> SKALLKGVRDFNPISACVCLLENSSDGH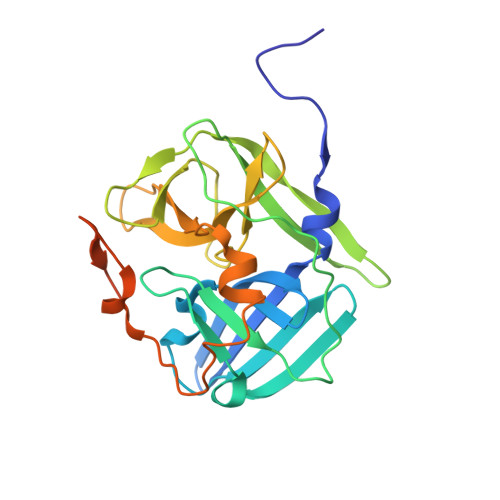SERLFGIGFGPYIIANQHLFRRNNGELTIKTMHGEFAVANSTQLQMKPVEGRDIIVIKMAKDFPPFPQKLKFRQPTIKDRVCMVSTNFQQKSVSSLVSESSHIVHKEDTSFWQHWITTKDGQAGSPLVSIIDGNILGIHSLTHTTNGSNYFVEFPEKFVATYLDAADGWCKNWKFNADKISWGSFTLVEDAPEDDFMAKKTVAAIMDDLVRTQ>[2x]RCLFVCRHGERMDVVFGKYWLS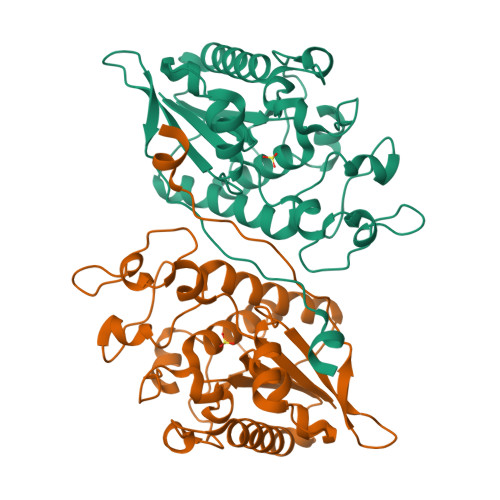QCFDAKGRYIRTNLNMPHSLPQRSGGFRDYEKDAPITVFGCMQARLVGEALLESNTVIDHVYCSPSLRCVQTAHNILKGLQQDNHLKIRVEPGLFEWTKWVAGSTLPAWIPPSELAAANLSVDTTYRPHIPVSKLAISESYDTYINRSFQVTKEIISECKSKGNNILIVAHASSLEACTCQLQGLSPQNSKDFVQMVRKIPYLGFCSCEELGETGIWQLTDPPILPLTHGPTGGFNWRETLL> MSGHHHHHHA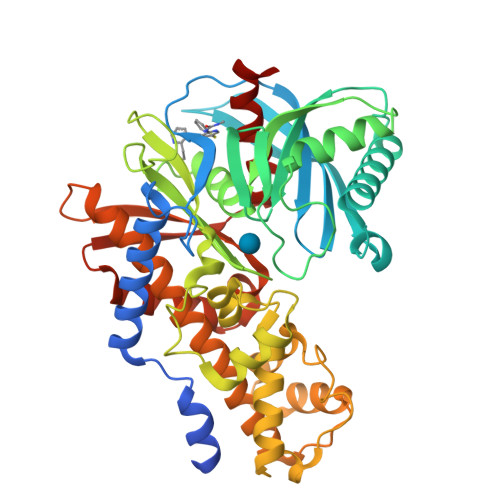SSGLVPRGSMALTLVEQILAEFQLQEEDLKKVMRRMQKEMDRGLRLETHEEASVKMLPTYVRSTPEGSEVGDFLSLDLGGTNFRVMLVKVGEGEEGQWSVKTKHQMYSIPEDAMTGTAEMLFDYISECISDFLDKHQMKHKKLPLGFTFSFPVRHEDIDKGILLNWTKGFKASGAEGNNVVGLLRDAIKRRGDFEMDVVAMVNDTVATMISCYYEDHQCEVGMIVGTGCNACYMEEMQNVELVEGDEGRMCVNTEWGAFGDSGELDEFLLEYDRLVDESSANPGQQLYEKLIGGKYMGELVRLVLLRLVDENLLFHGEASEQLRTRGAFETRFVSQVESDTGDRKQIYNILSTLGLRPSTTDCDIVRRACESVSTRAAHMCSAGLAGVINRMRESRSEDVMRITVGVDGSVYKLHPSFKERFHASVRRLTPSCEITFIESEEGSGRGAALVSAVACKKACMLGQ> MRALAELLSDTTERQQALADEVGSEVTGSLDDLIVNLVSQQWRRPPSARNGMSVEVLIEMLPDGTITNASVSRSS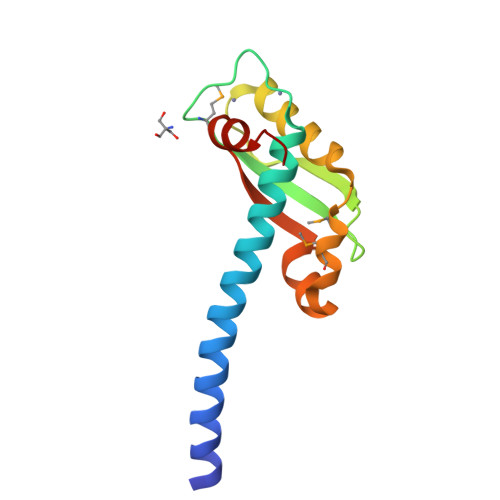GDKPFDSSAVAAVRNVGRIPEMQQLPRATFDSLYRQRRIIFKPEDLSLHHHHHH>MSAFQAFVVNKTETEFTAGV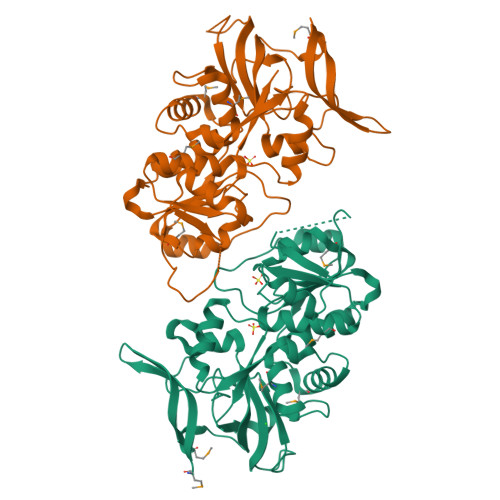QTISMDDLPEGDVLVRVHYSSVNYKDGLASIPDGKIVKTYPFVPGIDLAGVVVSSQHPRFREGDEVIATGYEIGVTHFGGYSEYARLHGEWLVPLPKGLTLKEAMAIGTAGFTAALSIHRLEEHGLTPERGPVLVTGATGGVGSLAVSMLAKRGYTVEASTGKAAEHDYLRVLGAKEVLAREDVMAERIRPLDKQRWAAAVDPVGGRTLATVLSRMRYGGAVAVSGLTGGAEVPTTVHPFILRGVSLLGIDSVYCPMDLRLRIWERLAGDLKPDLERIAQEISLAELPQALKRILRGELRGRTVVRLA[2x]> TNCDREPIHIPGAIQPHGVLLVLSEPGLVLTHASENA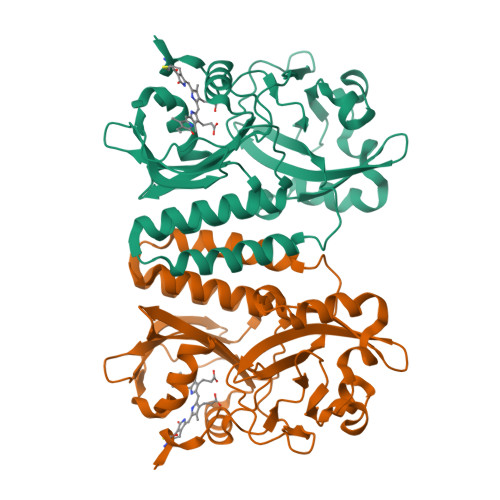PAVLGNSAEQLLGAPLGHFIEPSVREPLEADLRSARLKQLNPLKVVWRVDGVDRFFDGIAHRHQGRLILELEPSSHREAVPFLSFFHAVRDGLSRLRDARDLQELCEAVVQEVRGLTGFDRAIIYRFDAEWNGSVIAEARDARADPYLGLHFPASDIPRQARELYQLNWLRIIPTIDYQPARVRALPGHGEPLDLSFSVLRSVSPIHLEYLHNMGVQASMSISLMKDGKLWGLISCHQVSGTRYVPYEVRTACEFLGEVMSSLLAA5,10-METHYLENE-6-HYDROFOLIC ACID | C20 H21 N7 O6 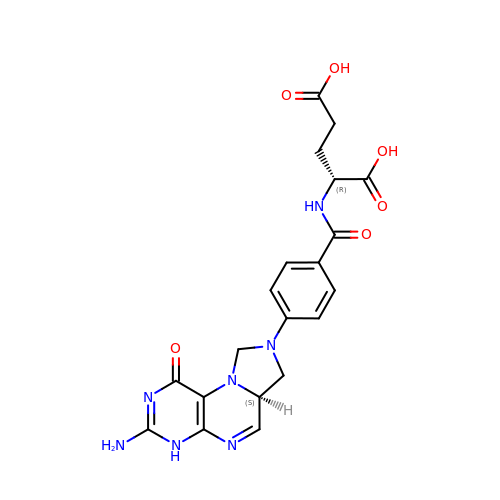| BHJAPJNOACHPNI-CHWSQXEVSA-N>[2x]MPVRKAKAVWEGGLRQGKGVMELQSQAFQGPYSYPSRFEEGEGTNPEELIAAAHAGCFSMALAASLEREGFPPKRVSTEARVHLEVVDGKPTLTRIELLTEAE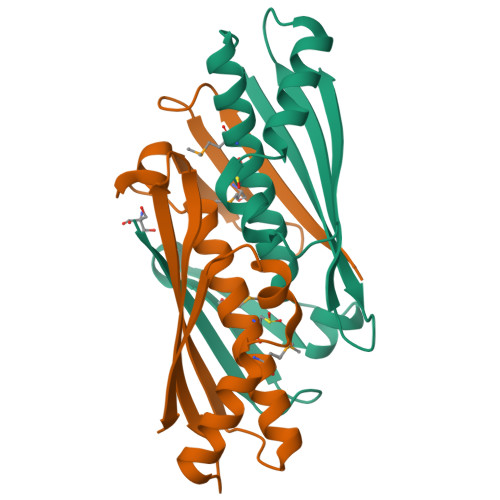VPGISSEKFLEIAEAAKEGCPVSRALAGVKEVVLTARLV>DMDLDSYQIALEEVLTWLLSAEDTFQEQDDISDDVEDVKEQFATHETFMMELSAHQSSVGSVLQAGN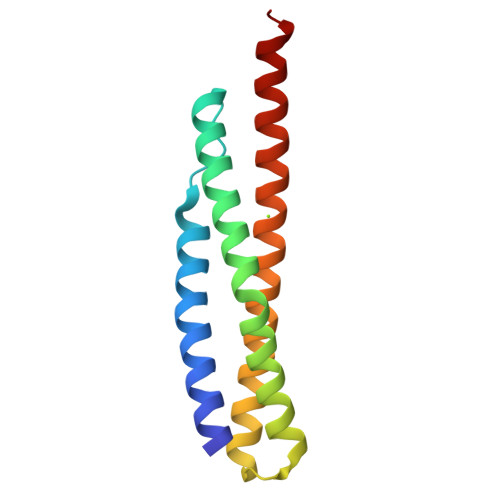QLMTQGTLSDEEEFEIQEQMTLLNARWEALRVESMERQSRLHDALMELQKKQLQQL[2x]>[3x]NVEEETKYIELMIVNDHLMFKKHRLSVVHTNTYAKSVVNMADLIYKDQLKTRIVLVAMETWATDNKFAISENPLITLREFMKYRRDFIKEKSDAVHLFSGSQFESSRSGAAYIGGICSLLKGGGVNEFGKTDLMAVTLAQSLAHNIGIISDKRKLASGECKCEDTWSGCIMGDTGYYLPKKFTQCNIEEYHDFLNSGGGACLFNKPSKLLDPPECGNGFIETGEECDCGTPAECVLEGAECCKKCTLTQDSQCSDGLCCKKCKFQPMGTVCREAVNDCDIRETCSGNSSQCAPNIHKMDGYSCDGVQGICFGGRCKTRDRQCKYIWGQKVTASDKYCYEKLNIEGTEKGNCGKDKDTWIQCNKRDVLCGYLLCTNIGNIPRLGELDGEITSTLVVQQGRTLNCSGGHVKLEEDVDLGYVEDGTPCGPQMMCLEHRCLPVASFNFSTCLSSKEGTICSGNGVCSNELKCVCNRHWIGSDCNTYFPHNDDAKTGITLSG;>[3x]DAAQPARRARRTYEAYPAKPKCPAVCTCTKDNALCENARSIPRTVPPDVISLSFVRSGFTEISEGSFLFTPSLQLLLFTSNSFDVISDDAFIGLPHLEYLFIENNNIKSISRHTFRGLKSLIHLSLANNNLQTLPKDIFKGLDSLTNVDLRGNSFNCDCKLKWLVEWLGHTNATVEDIYCEGPPEYKKRKINSLSSKDFDCIITEFAKSQDLPYQSLSIDTFSYLNDEYVVIAQPFTGKCIFLEWDHVEKTFRNYDNITGTSTVVCKPIVIETQLYVIVAQLFGGSHIYKRDSFANKFIKIQDIEILKIRKPNDIETFKIENNWYFVVADSSKAGFTTIYKWNGNG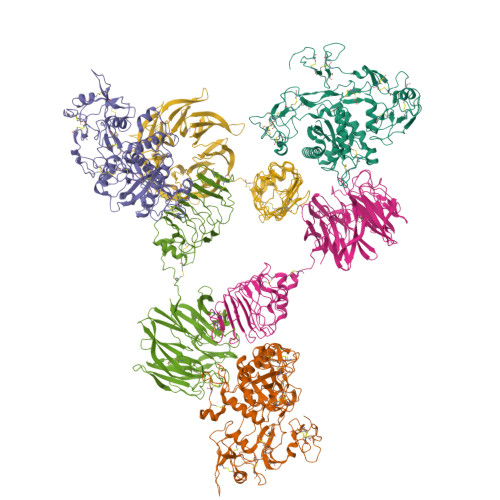FYSHQSLHAWYRDTDVEYLEIVRTPQTLRTPHLILSSSSQRPVIYQWNKATQLFTNQTDIPNMEDVYAVKHFSVKGDVYICLTRFIGDSKVMKWGGSSFQDIQAMPSRGSMVFQPLQINNYQYAILGSDYSFTQVYNWDAEKAKFVKFQELNVQAPRSFTHVSINKRNFLFASSFKGNTQIYKHVIVDLSAKHHHHHH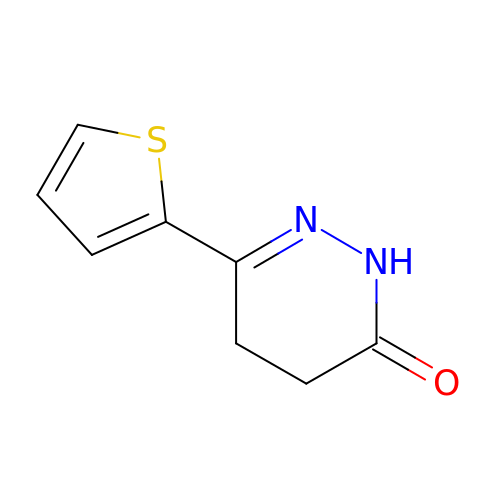3-thiophen-2-yl-4,5-dihydro-1~{H}-pyridazin-6-one | C8 H8 N2 O S | SLIODHPLYGIMCY-UHFFFAOYSA-N3-[[4-imidazol-1-yl-6-[(3~{S})-3-oxidanylpiperidin-1-yl]-1,3,5-triazin-2-yl]amino]-4-methyl-~{N}-[3-(trifluoromethyl)phenyl]benzamide 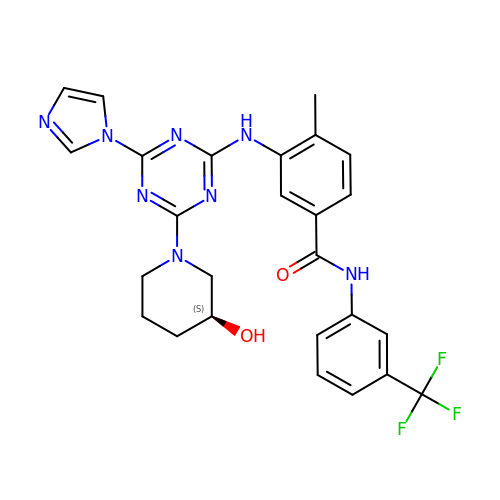| C26 H25 F3 N8 O2 | JHUYRHDBWXUNON-FQEVSTJZSA-N>STFSSLVIGSNTFIPTAPGYYSLSTRGFSDPRNQIKISGGKFNAKTGRVTAAVSRLWETDVTVAGLPVRSAAEVAIIMTLGRGITATNADVLLSDLNTLLD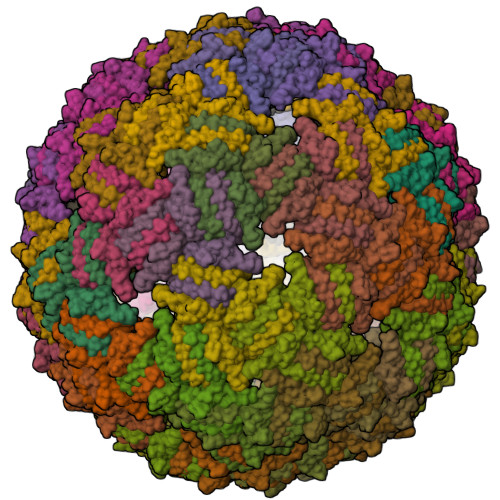PARLDQILQGGF[360x]NICOTINAMIDE 8-BROMO-ADENINE DINUCLEOTIDE PHOSPHATE | C21 H27 Br N7 O17 P3 | 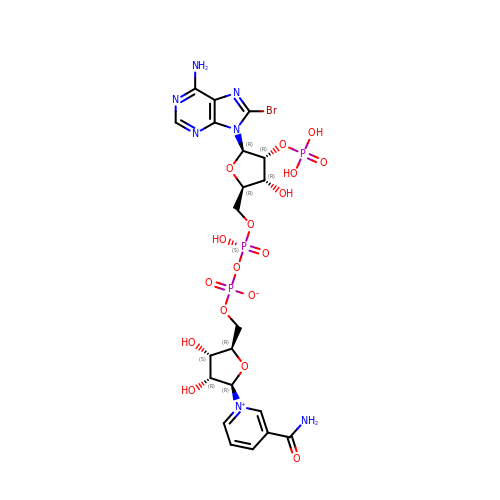MDKMTCCUJSRQGW-NAJQWHGHSA-N>[2x]SNAMRAHTLSRQLREGNLFAEQCPSREVLKHVTSRWGVLILVALRDGTHRFSDLRRKMGGVSEKMLAQSLQALEQDGFLNRVSYPVVPPHVEYSLTPLGEQVSDKVAALADWIE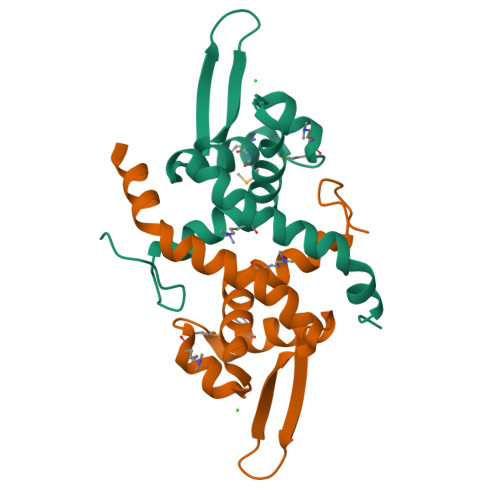LNLPQVLAQRERLSDGG> GSRAYSFKVVLLGEGCVGKTSLVLRYCENKFNDKHITTLQASFLTKKLNIGGKRVNLAIWDTAGQERFHALGPIYYRDSNGAILVYDITDEDSFQKVKNWVKELRKMLGNEICLCIVGNKIDLEKERHVSIQEAESYAESVGAKH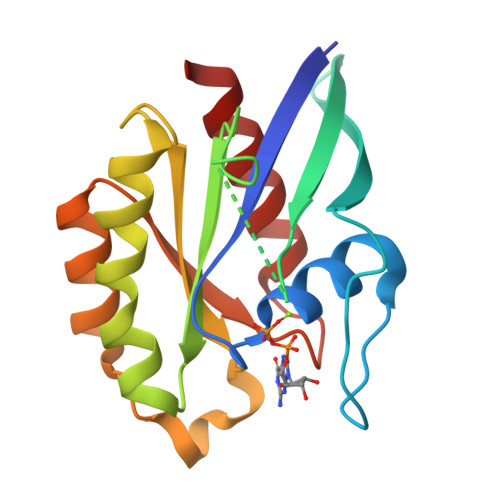YHTSAKQNKGIEELFLDLCKRMIET>MEGTGVVAVYGNGAITEAKKSPFSVKVGLAQMLRGGVIMDVVNAEQARIAEEAGACAVMALERVPADIRAQGGVARMSDPQMIKEIKQAVTIPVMAKARIGHFVEAQILEAIGIDYIDESEVLTLADEDHHINKHNFRIPFVCGCRNLGEALRRIREGAAMIRTKG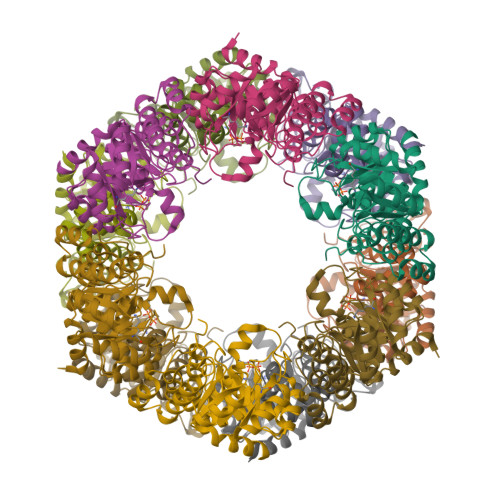EAGTGNIIEAVRHVRSVNGDIRVLRNMDDDEVFTFAKKLAAPYDLVMQTKQLGRLPVVQFAAGGVATPADAALMMQLGCDGVFVGSGIFKSGDPARRARAIVQAVTHYSDPEMLVEVSCGLGEAMVGINLNDEKVERFANRSEEHHHHHH[4x]>GPMPGKSVVARVAEARPEDVGKRIVRMDKAERAKLGVSVG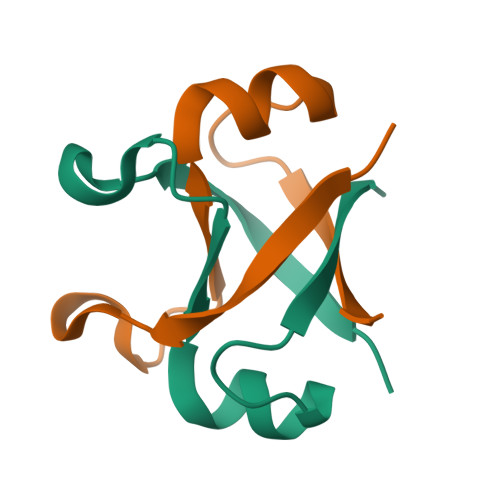DVVEVKKV[2x]3-{1-[(3R)-1-acryloylpiperidin-3-yl]-4-amino-1H-pyrazolo[3,4-d]pyrimidin-3-yl}-N-(3-tert-butylphenyl)benzamide | C30 H33 N7 O2 | 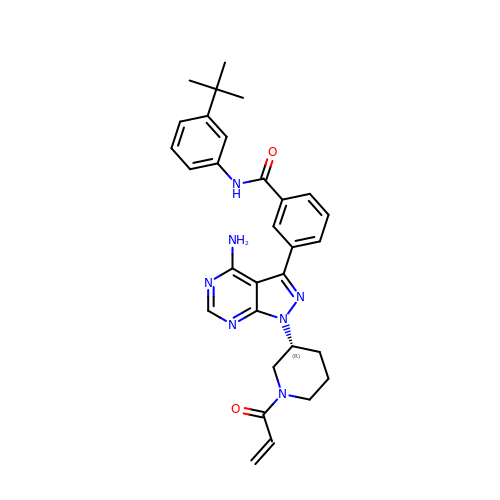RMAUIYTVKFMOGP-HSZRJFAPSA-N>[8x]SNAMST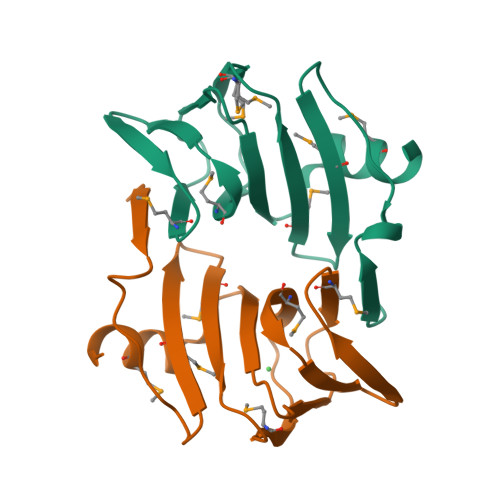GEQREFAPAFYDLTEVRSFSPLPGFAMQAIQGKNLMLNWVRIEPNTEMPAHEHPHEQAGVMLEGTLELTIGEETRVLRPGMAYTIPGGVRHRARTFEDGCLVLDIFSPPREDYARMAEDA> GSHMRQLKIVVLGDGASGKTSLTTCFAQETFGKQYKQTIGLDFFLRRITLPGNLNVTLQIWDIGGQTIGGKMLDKYIYGAQGVLLVYDITNYQSFENLEDWYTVVKKVSEE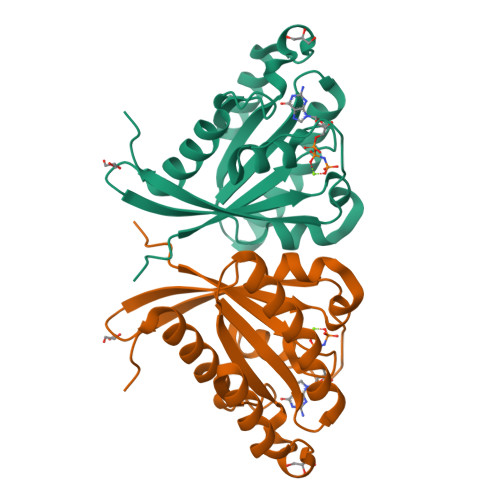SETQPLVALVGNKIDLEHMRTIKPEKHLRFCQENGFSSHFVSAKTGDSVFLCFQKVAAEILGIKLNK> MRLPDPYTNPEYPGLGFESVNLVDNDPMIRDELPNGKVKEVKISAQYWGINISYPELFPDEYAFLDSRLLEYKRTGDYLDVLLPQYEAFRVRGDTKS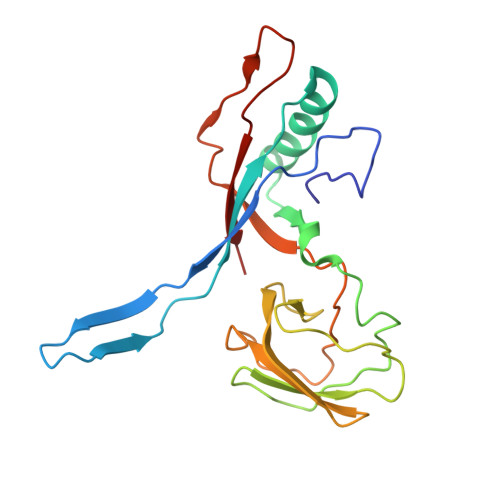VTIPAGQKGSQIILNTNGTLTGQPKAGDLFKLSTHPKVYKITNFSSSGNVWNISLYPDLFITTTGSEKPVFNGILFRTKLMNGDSFGSTLNNNGTYSGISLSLRESL> LPCVPFSVAKSVKSLYLGRMFSGTPVIRLRFKRLQPTRLVAEFDFRTFDPEGILLFAGGHQDSTWIVLALRAGRLELQLRYNGVGRVTSSGPVINHGMWQTISVEELARNLVIKVNRDAVMKIAVAGD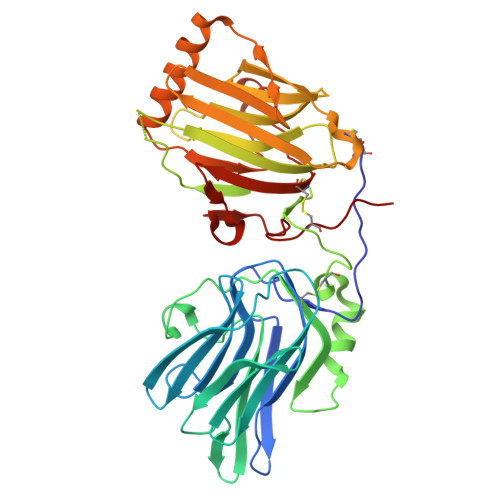LFQPERGLYHLNLTVGGIPFHEKDLVQPINPRLDGCMRSWNWLNGEDTTIQETVKVNTRMQCFSVTERGSFYPGSGFAFYSLDYMRTPLDVGTESTWEVEVVAHIRPAADTGVLFALWAPDLRAVPLSVALVDYHSTKKLKKQLVVLAVEHTALALMEIKVCDGQEHVVTVSLRDGEATLEVDGTRGQSEVSAAQLQERLAVLERHLRSPVLTFAGGLPDVPVTSAPVTAFYRGCMTLEVNRRLLDLDEAAYKHSDITAHSCPPVEP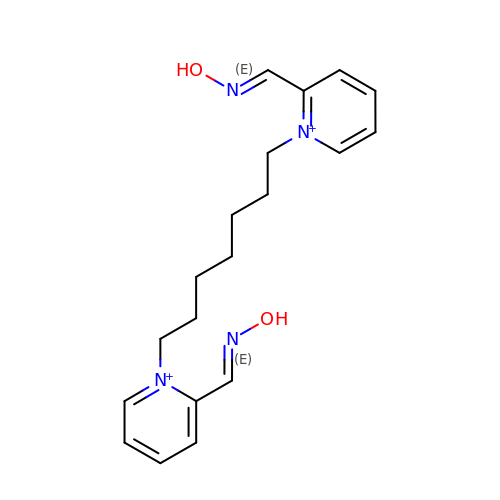1,7-HEPTYLENE-BIS-N,N'-SYN-2-PYRIDINIUMALDOXIME | C19 H26 N4 O2 | NJSMUQMHXZRXQC-UHFFFAOYSA-P>[2x]MSCQGPVCTNLGLKPGQRLTVKGIIAPNAKSFVMNLGKDSTHLGLHFNPRFDAHGDVNLIVCNSKKMEEWGTEQRETVFPFQKGAPIEIT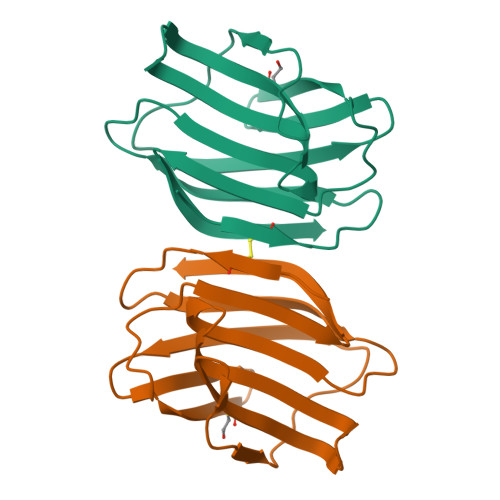FSINPSDLTVHLPGHQFSFPNRLGLSVFDYFDTHGDFTLRSVSWE>MGHHHHHHSQDPNSNVTLTAVKKAFPDALTNAELVAMVSKRLSQFGYHKYNTLLATS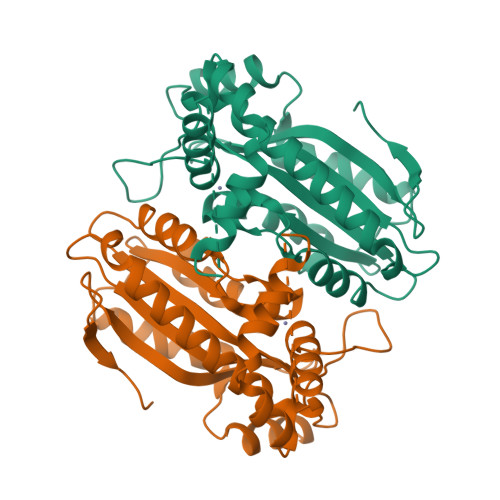LCSDEVTRPLEQDFGEVYGKHFTMGGLAGFPFGGLTGFGAMAGAIPDGGSCLLIYGSHVGVSWEGKWGTVARRGREKGGACCGSAVAAAQAVTQAYQATLDESSSSSSSSATSTPVYRYSNDPLDAQQGYVRDMLRPYAATLSEAEDVMVTLPVSVYDAQQKLVTRILDEGSNHIDGDGQIAVVGGIQINTPKEMSDFFVVRRFCIRDSSGNMVENFMPLTAGRE[2x]>MKISFASFKPMHDEIEYEIKFKFEEIYKRNWFILGDEDKKFEQEFADYCNVNYCIGCGNGLDALHLILKGYDIGFGDEVIVPSNTFIATALAVSYTGAKPIFVEPDIRTYNIDPSLIESAITEKTKAIIAVHLY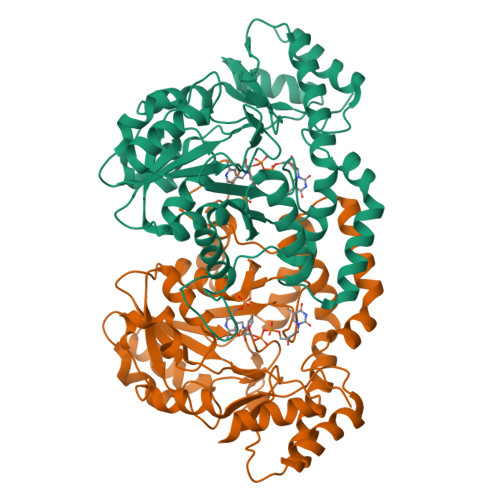GQPADMDEIKRIAKKYNLKLIEDAAQAHGSLYKGMKVGSLGDAAGFSFYPAKNLGSLGDGGAVVTNDKDLAEKIKALSNYGSEKKYHHIYKGFNSRLDELQAGFLRVKLKYLDKWNEERRKIAQKYIAGINNPNVIIPVEADYAKHVWYTFVIRSEKRDELQKYLNNNGIGTLIHYPIPIHLQQAYKDLGFKTGNFPIAEKIANEILSIPIWYGMKNEEIEYVIDKINAWKLEHHHHHH[2x]 4-methylisoleucine | C7 H15 N O2 | 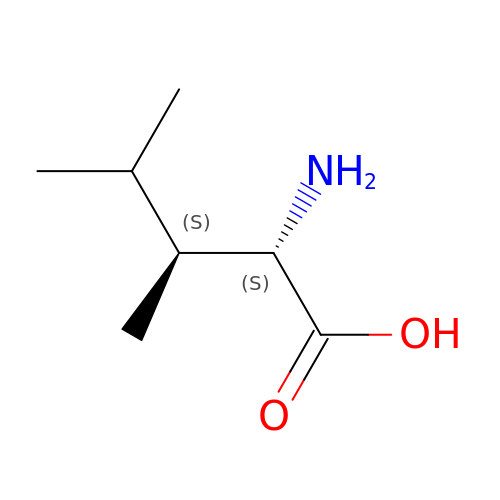VFEDCKXLINRKLV-WDSKDSINSA-N> GPDSMEEETHTDAKIRAENGTGSSPRGPGCSLRHFACEQNLLSRPDGSASFLQGDTSVLAGVYGPAEVKVSKEIFNKATLEVILRPKIGLPGVAEKSRERLIRNTCEAVVLGTLHPRTSITVVLQVVSDAGSLLACCLNAACMALVDAGVPMRALFCGVACALDSDGTLV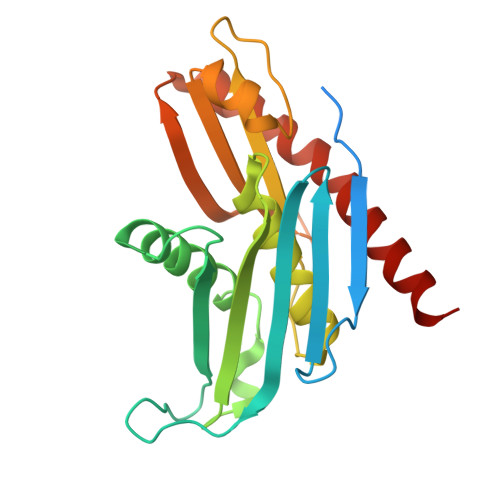LDPTSKQEKEARAVLTFALDSVERKLLMSSTKGLYSDTELQQCLAAAQAASQHVFRFYRESLQRRYSKS(3E)-3-({4-[(2-carboxyethyl)carbamoyl]phenyl}hydrazono)-6-oxocyclohexa-1,4-diene-1-carboxylic 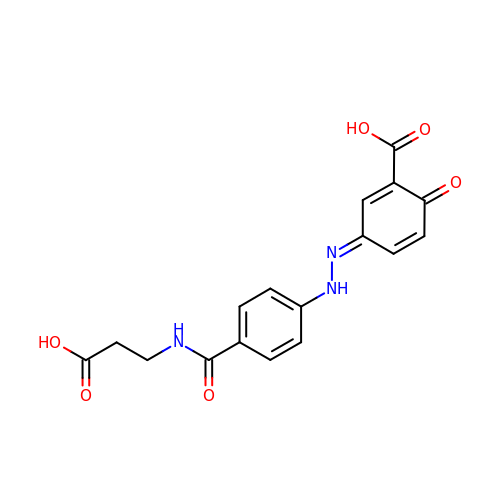acid | C17 H15 N3 O6 | KONZVQJABTUMFX-UDWIEESQSA-N> SHLGTYGVFTNAA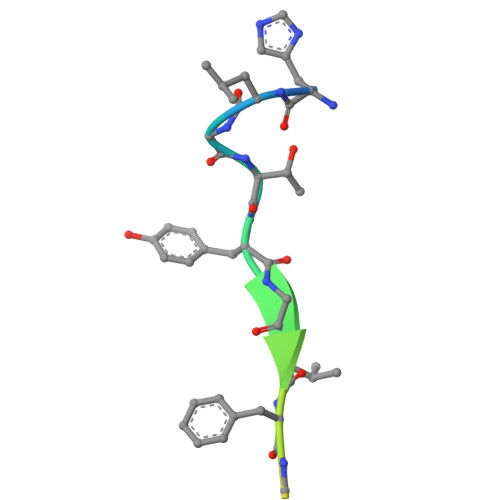FDPSP> SLEST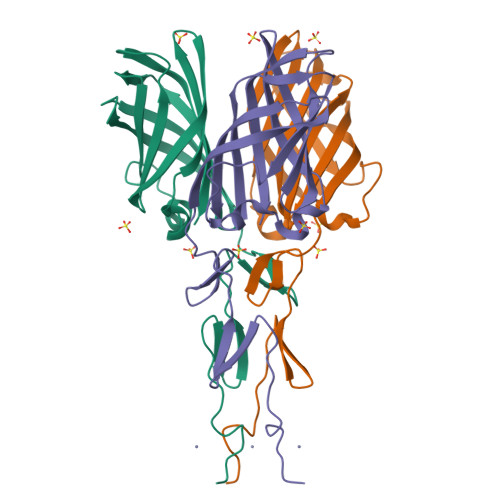ASHGLSFSPPLSVADGVVSLDMDPYFCSQRVSLTSYSAEAQLMQFRWMARGTNGSSDTIDMTVNAHCHGRRTDYMMSSTGNLTVTSNVVLLTFDLSDITHIPSDLARLVPSAGFQAASFPVDVSFTRDSATHAYQAYGVYSSSRVFTITFPTGGDGTANIRSLTVRTGIDT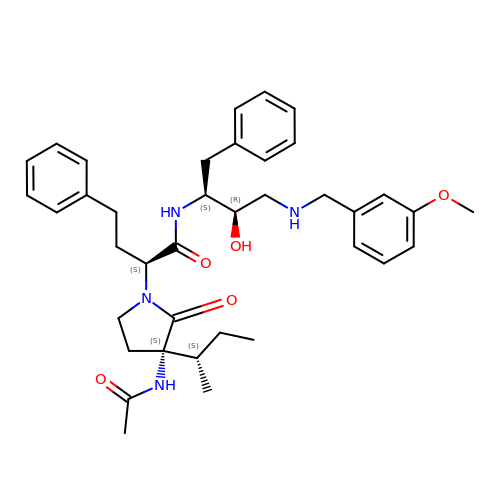(2S)-2-{(3S)-3-(acetylamino)-3-[(2S)-butan-2-yl]-2-oxopyrrolidin-1-yl}-N-{(2S,3R)-3-hydroxy-4-[(3-methoxybenzyl)amino]-1-phenylbutan-2-yl}-4-phenylbutanamide | C38 H50 N4 O5 | SMPAHDBHYSCFQF-SXXDCNOLSA-N The Origin Recognition Complex (ORC) binds to sites in chromosomes to specify the location of origins of DNA replication. The S. cerevisiae ORC binds to specific DNA sequences throughout the cell cycle but becomes active only when it binds to the replication initiator Cdc6. The ORC–Cdc6 complex (product 1) assembles in step 1 around origin DNA and with the help of another replication initiator protein, Cdt1, it recruits the Mcm2-7 hexamer to the origin in step 2. Here we report the cryo-EM structure at 3.3 Å resolution of the yeast ORC–Cdc6 bound to an 85-bp ARS1 origin DNA.

The six AAA+−containing subunits (Orc1-5 and Cdc6) of ORC–Cdc6–DNA are arranged in a two-tiered, spiral structure that encircles the origin DNA, with the top tier formed by the AAA+ domains and the lower tier by the WHD domains. On the top tier, the gap between the Orc1 AAA+ and the Orc2 AAA+-like domain vacated by the Orc2 WHD became occupied by the Cdc6 AAA+ domain, and the AAA+ domains of Orc1-5 and Cdc6 form a nearly flat ring that encircles the ACS region of the origin DNA. Specifically, the Orc2 WHD was evicted from the center of the 5-membered AAA+ ring in the structure of ORC–DNA and was replaced by the Cdc6 AAA+ domain, forming the closed ring of six AAA+ domains around the ACS element in the ORC–Cdc6–DNA structure. Indeed, four ATPγS molecules and their associated Mg2+ were identified in the AAA+ domains of Orc1, Orc4, Orc5, and Cdc6. Therefore, the ORC–Cdc6 complex bound and stabilized 50 bp of the ARS1 origin DNA, which is 9 bp longer than that of ORC alone, which stabilized 41 bp of the ARS305 origin. Cdc6 was found to interact extensively with dsDNA in a bipartite manner, with the ISM of its AAA+ domain binding to the middle of the ACS sequence and the WHD hairpin motif binding to the intervening region between the A and B1 elements. The positively charged residues K477, K479, K481, and K483 in the Cdc6 WHD hairpin motif interact with the ACS phosphate backbone, but do not insert into the DNA groove, and therefore most likely increases the affinity of the ORC–Cdc6 complex for DNA. Our structure shows that Cdc6 binding stabilizes the Orc6 TFIIB-B domain, which in turn binds and stabilizes the eight nucleotides following the B1 element. We found that Cdc6 binding shifted a helix-turn-helix (HTH) motif in Orc1 by about 5 Å to form a part of the ATP binding site of Cdc6. In fact, the Orc1 Arg-616 points to the γ-phosphate and serves as the arginine finger in trans for the ATP molecule in the Cdc6 pocket.

> MAKTLKDLQGWEIITTDEQGNIIDGGQKRLRRRGAKTEHYLKRSSDGIKLGRGDSVVMHNEAAGTYSVYMIQELRLNTLNNVVELWALTYLRWFEVNPLAHYRQFNPDANILNRPLNYYNKLFSETANKNELYLTAELAELQLFNFIRVANVMDGSKWEVLKGNVDPERDFTVRYICEPTGEKFVDINIEDVKAYIKKVEPREAQEYLKDLTLPSKKKEIKRGPQKKDKATQTAQISDAETRATDITDNEDGNEDESSDYESPSDIDVSEDMDSGEISADELEEEEDEEEDEDEEEKEARHTNSPRKRGRKIKLGKDDIDASVQPPPKKRGRKPKDPSKPRQMLLISSCRANNTPVIRKFTKKNVARAKKKYTPFSKRFKSIAAIPDLTSLPEFYGNSSELMASRFENKLKTTQKHQIVETIFSKVKKQLNSSYVKEEILKSANFQDYLPARENEFASIYLSAYSAIESDSATTIYVAGTPGVGKTLTVREVVKELLSSSAQREIPDFLYVEINGLKMVKPTDCYETLWNKVSGERLTWAASMESLEFYFKRVPKNKKKTIVVLLDELDAMVTKSQDIMYNFFNWTTYENAKLIVIAVANTMDLPERQLGNKITSRIGFTRIMFTGYTHEELKNIIDLRLKGLNDSFFYVDTKTGNAILIDAAGNDTTVKQTLPEDVRKVRLRMSADAIEIASRKVASVSGDARRALKVCKRAAEIAEKHYMAKHGYGYDGKTVIEDENEEQIYDDEDKDLIESNKAKDDNDDDDDNDGVQTVHITHVMKALNETLNSHVITFMTRLSFTAKLFIYALLNLMKKNGSQEQELGDIVDEIKLLIEVNGSNKFVMEIAKTLFQQGSDNISEQLRIISWDFVLNQLLDAGILFKQTMKNDRICCVKLNISVEEAKRAMNEDETLRNL;> MLNGEDFVEHNDILSSPAKSRNVTPKRVDPHGERQLRRIHSSKKNLLERISLVGNERKNTSPDPALKPKTPSKAPRKRGRPRKIQEELTDRIKKDEKDTISSKKKRKLDKDTSGNVNEESKTSNNKQVMEKTGIKEKREREKIQVATTTYEDNVTPQTDDNFVSNSPEPPEPATPSKKSLTTNHDFTSPLKQIIMNNLKEYKDSTSPGKLTLSRNFTPTPVPKNKKLYQTSETKSASSFLDTFEGYFDQRKIVRTNAKSRHTMSMAPDVTREEFSLVSNFFNENFQKRPRQKLFEIQKKMFPQYWFELTQGFSLLFYGVGSKRNFLEEFAIDYLSPKIAYSQLAYENELQQNKPVNSIPCLILNGYNPSCNYRDVFKEITDLLVPAELTRSETKYWGNHVILQIQKMIDFYKNQPLDIKLILVVHNLDGPSIRKNTFQTMLSFLSVIRQIAIVASTDHIYAPLLWDNMKAQNYNFVFHDISNFEPSTVESTFQDVMKMGKSDTSSGAEGAKYVLQSLTVNSKKMYKLLIETQMQNMGNLSANTGPKRGTQRTGVELKLFNHLCAADFIASNEIALRSMLREFIEHKMANITKNNSGMEIIWVPYTYAELEKLLKTVLNTL;> MSDLNQSKKMNVSEFADAQRSHYTVYPSLPQSNKNDKHIPFVKLLSGKESEVNVEKRWELYHQLHSHFHDQVDHIIDNIEADLKAEISDLLYSETTQKRRCFNTIFLLGSDSTTKIELKDESSRYNVLIELTPKESPNVRMMLRRSMYKLYSAADAEEHPTIKYEDINDEDGDFTEQNNDVSYDLSLVENFKRLFGKDLAMVFNFKDVDSINFNTLDNFIILLKSAFKYDHVKISLIFNINTNLSNIEKNLRQSTIRLLKRNYHKLDVSSNKGFKYGNQIFQSFLDTVDGKLNLSDRFVEFILSKMANNTNHNLQLLTKMLDYSLMSYFFQNAFSVFIDPVNVDFLNDDYLKILSRCPTFMFFVEGLIKQHAPADEILSLLTNKNRGLEEFFVEFLVRENPINGHAKFVARFLEEELNITNFNLIELYHNLLIGKLDSYLDRWSACKEYKDRLHFEPIDTIFQELFTLDNRSGLLTQSIFPSYKSNIEDNLLSWEQVLPSLDKENYDTLSGDLDKIMAPVLGQLFKLYREANMTINIYDFYIAFRETLPKEEILNFIRKDPSNTKLLELAETPDAFDKVALILFMQAIFAFENMGLIKFQSTKSYDLVEKCVWRGI;> MTISEARLSPQVNLLPIKRHSNEEVEETAAILKKRTIDNEKCKDSDPGFGSLQRRLLQQLYGTLPTDEKIIFTYLQDCQQEIDRIIKQSIIQKESHSVILVGPRQSYKTYLLDYELSLLQQSYKEQFITIRLNGFIHSEQTAINGIATQLEQQLQKIHGSEEKIDDTSLETISSGSLTEVFEKILLLLDSTTKTRNEDSGEVDRESITKITVVFIFDEIDTFAGPVRQTLLYNLFDMVEHSRVPVCIFGCTTKLNILEYLEKRVKSRFSQRVIYMPQIQNLDDMVDAVRNLLTVRSEISPWVSQWNETLEKELSDPRSNLNRHIRMNFETFRSLPTLKNSIIPLVATSKNFGSLCTAIKSCSFLDIYNKNQLSNNLTGRLQSLSDLELAILISAARVALRAKDGSFNFNLAYAEYEKMIKAINSRIPTVAPTTNVGTGQSTFSIDNTIKLWLKKDVKNVWENLVQLDFFTEKSAVGLRDNATAAFYASNYQFQGTMIPFDLRSYQMQIILQELRRIIPKSNMYYSWTQL;> MNVTTPEVAFREYQTNCLASYISADPDITPSNLILQGYSGTGKTYTLKKYFNANPNLHAVWLEPVELVSWKPLLQAIARTVQYKLKTLYPNIPTTDYDPLQVEEPFLLVKTLHNIFVQYESLQEKTCLFLILDGFDSLQDLDAALFNKYIKLNELLPKDSKINIKFIYTMLETSFLQRYSTHCIPTVMFPRYNVDEVSTILVMSRCGELMEDSCLRKRIIEEQITDCTDDQFQNVAANFIHLIVQAFHSYTGNDIFALNDLIDFKWPKYVSRITKENIFEPLALYKSAIKLFLSTDDNLSENGQGESAITTNRDDLENSQTYDLSIISKYLLIASYICSYLEPRYDASIFSRKTRIIQGRAAYGRRKKKEVNPRYLQPSLFAIERLLAIFQAIFPIQGKAESGSLSALREESLMKANIEVFQNLSELHTLKLIATTMNKNIDYLSPKVRWKVNVPWEIIKEISESVHFNISDYFSDIHE;> MSMQQVQHCVAEVLRLDPQEKPDWSSGYLKKLTNATSILYNTSLNKVMLKQDEEVARCHICAYIASQKMNEKHMPDLCYYIDSIPLEPKKAKHLMNLFRQSLSNSSPMKQFAWTPSPKKNKRSPVKNGGRFTSSDPKELRNQLFGTPTKVRKSQNNDSFVIPELPPMQTNESPSITRRKLAFEEDEDEDEEEPGNDGLSLKSHSNKSITGTRNVDSDEYENHESDPTSEEEPLGVQESRSGRTKQNKAVGKPQSELKTAKALRKRGRIPNSLLVKKYCKMTTEEIIRLCNDFELPREVAYKIVDEYNINASRLVCPWQLVCGLVLNCTFIVFNERRRKDPRIDHFIVSKMCSLMLTSKVDDVIECVKLVKELIIGEKWFRDLQIRYDDFDGIRYDEIIFRKLGSMLQTTNILVTDDQYNIWKKRIEMDLALTEPL;> MSAIPITPTKRIRRNLFDDAPATPPRPLKRKKLQFTDVTPESSPEKLQFGSQSIFLRTKALLQKSSELVNLNSSDGALPARTAEYEQVMNFLAKAISEHRSDSLYITGPPGTGKTAQLDMIIRQKFQSLPLSLSTPRSKDVLRHTNPNLQNLSWFELPDGRLESVAVTSINCISLGEPSSIFQKIFDSFQDLNGPTLQIKNMQHLQKFLEPYHKKTTFVVVLDEMDRLLHANTSETQSVRTILELFLLAKLPTVSFVLIGMANSLDMKDRFLSRLNLDRGLLPQTIVFQPYTAEQMYEIVIQKMSSLPTIIFQPMAIKFAAKKCAGNTGDLRKLFDVLRGSIEIYELEKRFLLSPTRGSLNSAQVPLTPTTSPVKKSYPEPQGKIGLNYIAKVFSKFVNNNSTRTRIAKLNIQQKLILCTIIQSLKLNSDATIDESFDHYIKAITKTDTLAPLQRNEFLEICTILETCGLVSIKKTKCKGKTKRFVDKIDVDLDMREFYDEMTKISILKPFLH>[2x]MAHHHHHHSAALEVLFQGPGPVSKIFFEQGTYQCLENCGTVALTIIRRGGDLTNTVFVDFRTEDGTANAGSDYEFTEGTVVFKPGETQKEIRVGIIDDDIF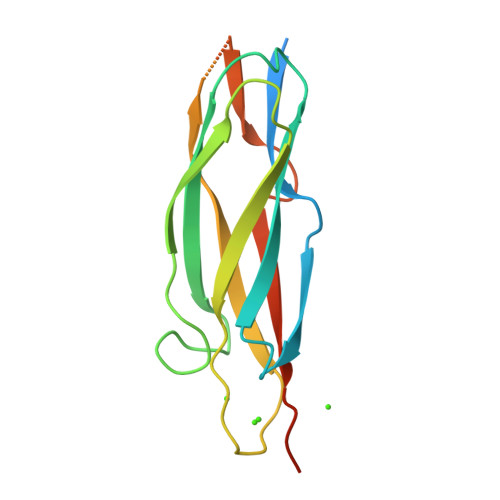EEDKNFLVHLSNVKVSSEASEDGILEANHVSALACLGSPSTATVTIFDDDHAGIFTFEE> MASEDHTEEINDKIYSLNYNELEVLAKNGETIENFVPKEG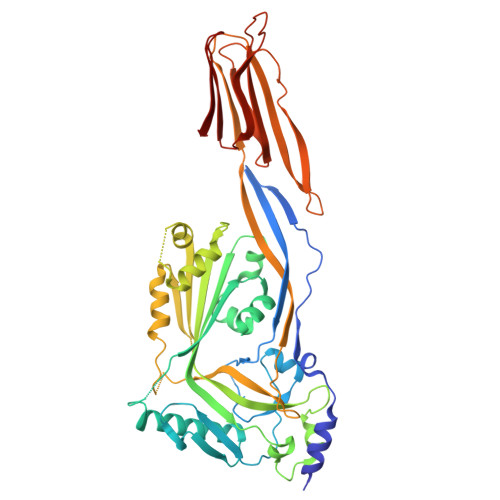VKKADKFIVIERKKKNINTTPVDISIIDSVTDRTYPAALQLANKGFTENKPDAVVTKRNPQKIHIDLPGMGDKATVEVNDPTYANVSTAIDNLVNQWHDNYSGGNTLPARTQYTESMVYSKSQIEAALNVNSKILDGTLGIDFKSISKGEKKVMIAAYKQIFYTVSANLPNNPADVFDKSVTFKELQRKGVSNEAPPLFVSNVAYGRTVFVKLETSSKSNDVEAAFSAALKGTDVKTNGKYSDILENSSFTAVVLGGDAAEHNKVVTKDFDVIRNVIKDNATFSRKNPAYPISYTSVFLKNNKIAGVNNRSEYVETTSTEYTSGKINLSHQGAYVAQYEILWDEINYDDKGKEVITKRRWDNNWYSKTSPFSTVIPLGANSRNIRIMARECTGLAWEWWRKVIDERDVKLSKEINVNISGSTLSPYGSITYK> VHFHPFGNVNFYEMDWSLKGDLWAHDPVIAKEGSRWYVFHTGSGIQIKT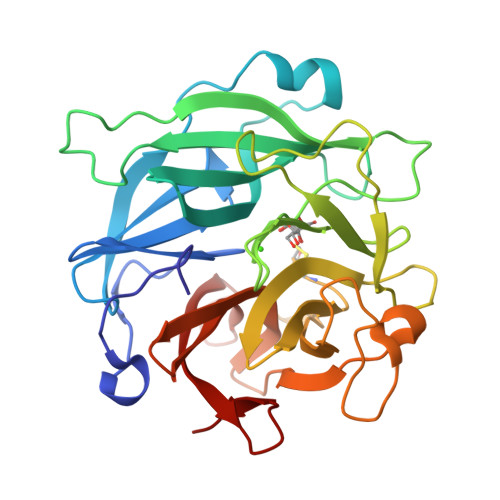SEDGVHWENMGWVFPSLPDWYKQYVPEKDEDHLWAPDICFYNGIYYLYYSVSTFGKNTSVIGLATNQTLDPRDPDYEWKDMGPVIHSTASDNYNAIDPNVVFDQEGQPWLSFGSFWSGIQLIQLDTETMKPAAQAELLTIASRGEEPNAIEAPFIVCRNGYYYLFVSFDFCCRGIESTYKIAVGRSKDITGPYVDKNGVSMMQGGGTILDEGNDRWIGPGHCAVYFSGVSAILVNHAYDALKNGEPTLQIRPLYWDDEGWPYLSV>MGEALKILNNIRTLRAQARECTLETLEEMLEKLEVVVNERREEESA[2x];>GSHMSDKPLTKTDYLMRLRRCQTIDTLERVIEKNKYELSDNELAVFYSAADHRLAELTMNKLYDKIPSSVWKFIR[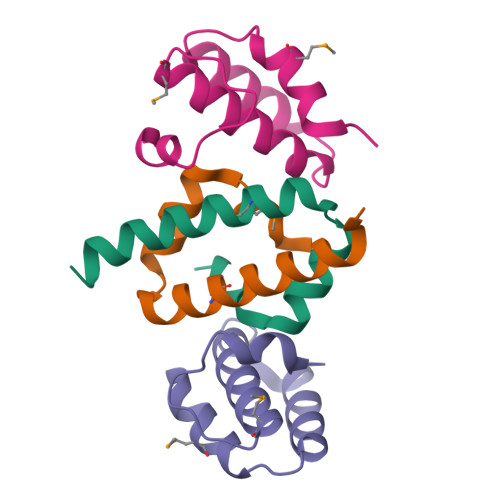2x]> ALPAKENEGCIVSVNSGKRYCLPVGQRSGYSLPDWIVGQEVYVDSGAKAKVLLSDWDNLSYNRIGEFVGNVNPADMKKVKAWNGQYLDFSKPRSMRVVYK;> AEAPTT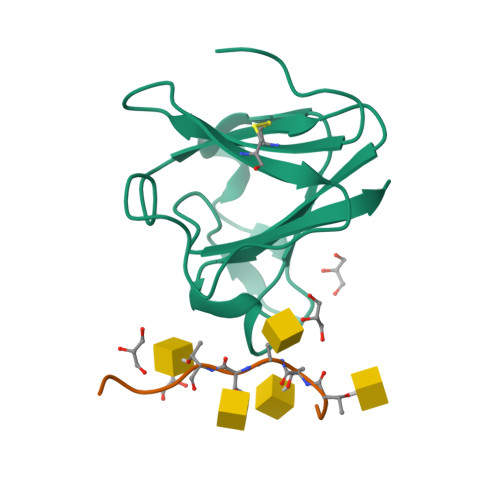STTSAPK>[2x]ADTYAATRYPVILVHGLAGTDKFANVVDYWYGIQSDLQSHGAKVYVANLSGFQSDDGPNGRGEQLLAYVKQVLAATGATKVNLIGHSQGGLTSRYVAAVAPQLVASVTTIGTPHRGSEFADFVQDVLKTDPTGLSSTVIAAFVNVFGTLVSSSHNTDQDALAALRTLTTAQTATYNRNFPSAGLGAPGSCQTGAATETVGGSQHLLYSWGGTAIQPTSTVLGVTGATDTSTGTLDVANVTDPSTLALLATGAVMINRASGQNDGLVSRCSSLFGQVISTSYHWNHLDEINQLLGVRGANAEDPVAVIRTHVNRLKLQGV;>[2x]GHHHHHHHHHHSSGHIEGRHMPAAPSPAPAGAVAGGPAA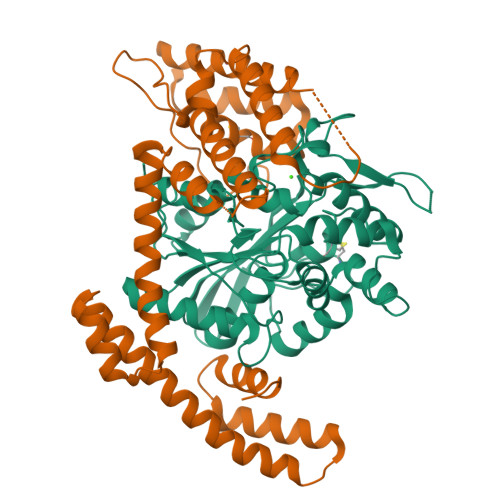GVPAAASGAAEAAMPLPAALPGALAGSHAPRLPLAAGGRLARTRAVREFFDYCLTAQGELTPAALDALVRREIAAQLDGSPAQAEALGVWRRYRAYFDALAQLPGDGAVLGDKLDPAAMQLALDQRAALADRTLGEWAEPFFGDEQRRQRHDLERIRIANDTTLSPEQKAARLAALDAQLTPDERAQQAALHAQQDAVTKIADLQKAGATPDQMRAQIAQTLGPEAAARAAQMQQDDEAWQTRYQAYAAERDRIAAQGLAPQDRDARIAQLRQQTFTAPGEAIRAASLDRGAG> MAQQTPLYEQHTLCGARMVDFHGWMMPLHYGSQIDEHHAVRTDAGMFDVSHMTIVDLRGSRTREFLRYLLANDVAKLTKSGKALYSGMLNASGGVIDDLIVYYFTEDFFRLVVNSATREKDLSWITQHAEPFGIEITVRDDLSMIAVQGPNAQAKAATLFNDAQRQAVEGMKPFFGVQAGDLFIATTGYTGEAGYEIALPNEKAADFWRALVEAGVKPCGLGARDTLRLEAGMNLYGQEMDETISPLAANMGWTIAWEPADRD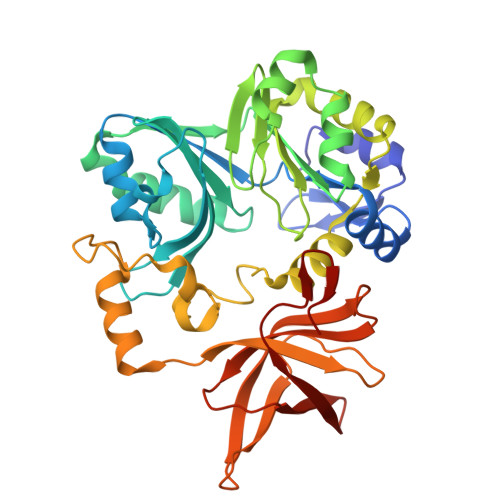FIGREALEVQREHGTEKLVGLVMTEKGVLRNELPVRFTDAQGNQHEGIITSGTFSPTLGYSIALARVPEGIGETAIVQIRNREMPVKVTKPVFVRNGKAVA>[10x]MSDDASTPAAERIPNKGKLAKDLNEVIRYTLW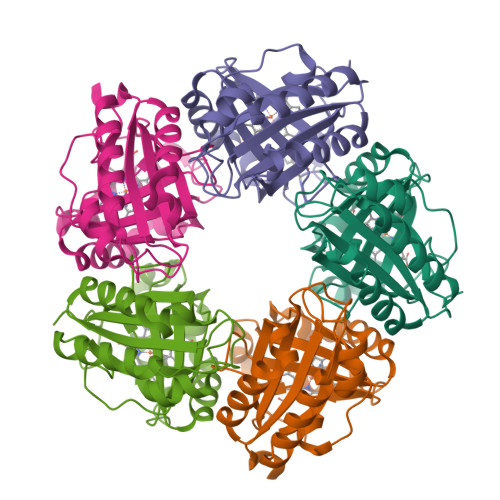SVFKLKDTLPEDRAGYADEVQELFDQLAAKDVTIRGTYDLSGLRADADLMIWWHAETADQLQEAYNLFRRTKLGRALEPVWSNMALHRPAEFNRSHIPAFLADETPRNYISVYPFVRSYDWYLLPDEDRRRMLADHGKMARGYPDVRANTVASFSLGDYEWILAFEADELHRIVDLMRHLRGSEARRHVREEIPFYTGRRKDIGELVAGLA>[6x]AHGRIELIIGPMFAGKTTELMRRVQRHKHAQRSCYIIKYTGDTRYSEGAITSHDQRALTANVSVSNLHDVGDEWRKYDVIAVDEGQFFPDVAAFCSKAADSGKVVIVSALD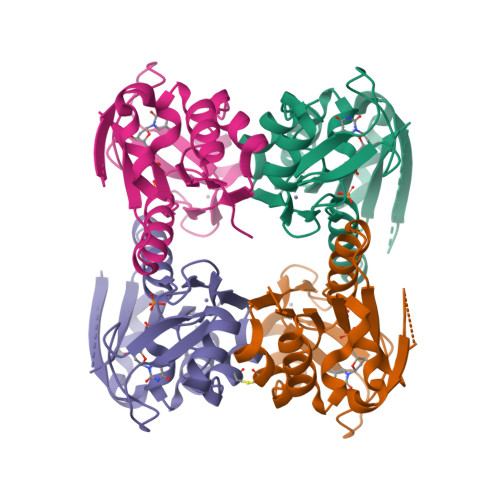ADYLQEPFEEICLLVSRADSVVKLSAVCMECHNRKASFTYRTVKSDERKLVGGSDMYMSVCRSCYETKRNMA(2E,4aR,7aS)-7a-(2,6-difluorophenyl)-6-(5-fluoro-4-methoxy-6-methylpyrimidin-2-yl)-2-imino-3-methyloctahydro-4H-pyrrolo[3,4-d]pyrimidin-4-one 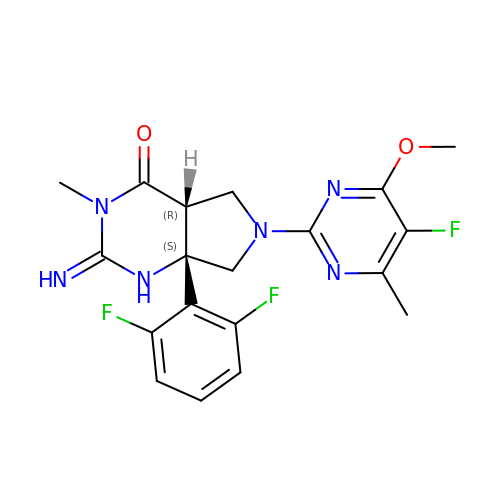| C19 H19 F3 N6 O2 | NAXGDHGFSCZYGN-OVWNDWIMSA-N> LNSCSMPLGMESKAISDAQITASSYFTNMFATWSPSKARLHLQGRSNAWRPQVNNPKEWLQVDFQKTMKVTGVTTQGVKSLLTSMYVKEFLISSSQDGHQWTLFFQNGKVKVFQGNQDSFTPVVNCLDP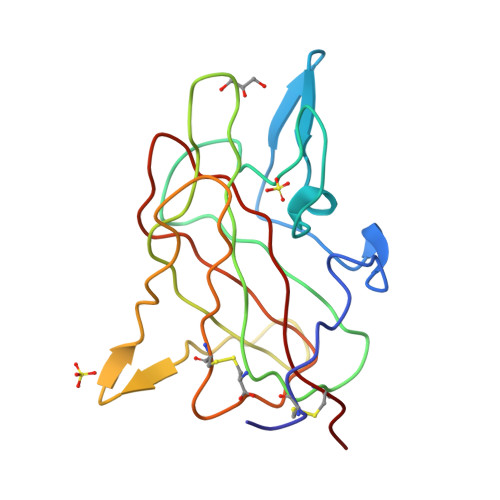PLLTRYLRIHPQSWVHQIALRMEVLGCEAQ N,3-dimethyl-N-[(pyridin-3-yl)methyl]-1,2-oxazole-5-carboxamide | 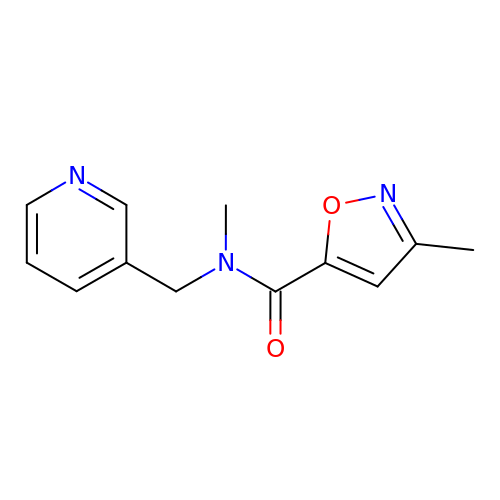C12 H13 N3 O2 | YRZCJLIACJLYBI-UHFFFAOYSA-N> MEQSVANLVDMRDVSFTRGNRCIFDNISLTVPRGKITAIMGPSGIGKTTLLRLIGGQIAPDHGEILFDGENIPAMSRSRLYTVRKRMSMLFQSGALFTDMNVFDNVAYPLREHTQLPAPLLHSTVMMKLEAVGLRGAAKLMPSELSGGMARRAALARAIALEPD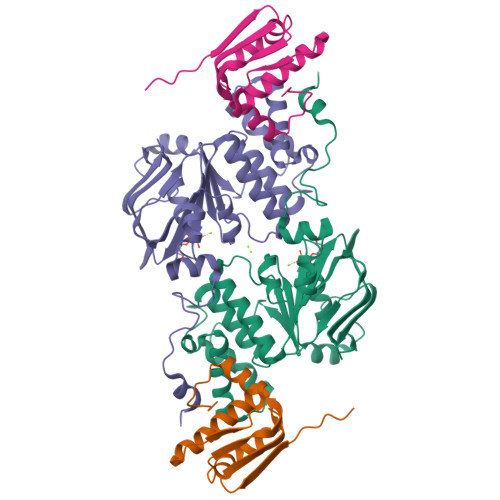LIMFDEPFVGQDPITMGVLVKLISELNSALGVTCVVVSHDVPEVLSIADHAWILADKKIVAHGSAQALQANPDPRVRQFLDGIADGPVPFRYPAGDYHADLLPGS;> MHHHHHHENLYFQSESLSWMQTGDTLALSGELDQDVLLPLWEMREEAVKGITCIDLSRVSRVDTGGLALLLHLIDLAKKQGNNVTLQGVNDKVYTLAKLYNLPADVLPR> MAQTVPYGIPLIKADKVQAQGFKGANVKVAVLDTGIQASHPDLNVVGGASFVAGEAYNTDGNGHGTHVAGTVAALDNTTGVLGVAPSVSLYAVKVLNSSGSGSYSGIVSGIEWATTNGMDVINMSLGGASGSTAMKQAVDNAYARGVVVVAAAGNSGSSGNTNTIGYPAKYDSVIAVGAVDSNSNRASFSSVGAELEVMAPGAGVYSTYPTNTYATLNGTSMASPHVAGAAALILSKHPNLSASQVR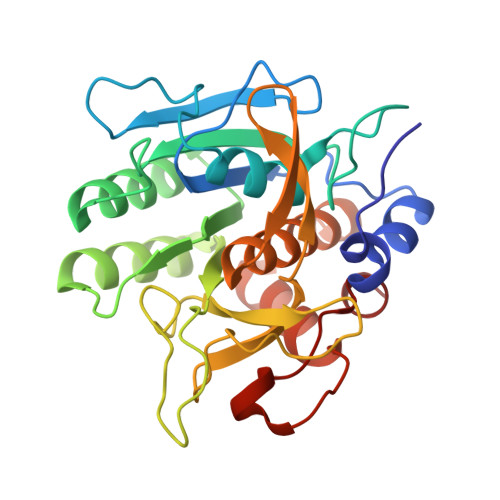NRLSSTATYLGSSFYYGKGLINVEAAAQ>MDSKHQCVKLNDGHFMPVLGFGTYAPPEVPRSKALEVTKLAIEAGFRHIDSAHLYNNEEQVGLAIRSKIADGSVKREDIFYTSKLWSTFHRPELVRPALENSLKKAQLDYVDLYLIHSPMSLKPGEELSPTDENGKVIFDIVDLCTTWEAMEKCKDAGLAKSIGVSNFNRRQLEMILNKPGLKYKPVCNQVECHPYFNRSKLLDFCKSKDIVL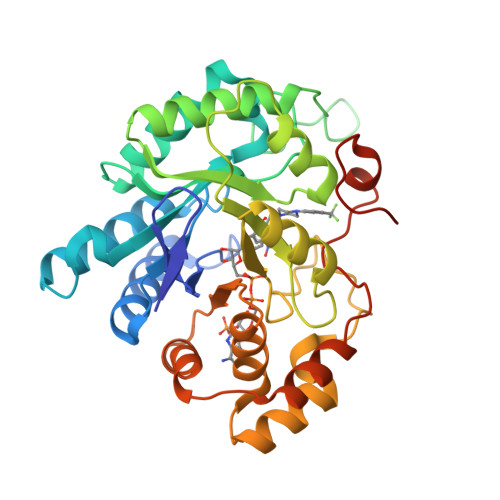VAYSALGSQRDKRWVDPNSPVLLEDPVLCALAKKHKRTPALIALRYQLQRGVVVLAKSYNEQRIRQNVQVFEFQLTAEDMKAIDGLDRNLHYFNSDSFASHPNYPYSDEYLEHHHHHH[2x]>MGSTRLRNASVWLCGLLCLLQVVPSINADVSGCKPGFSSAEYIFSVNRRELERGRKLGKVNFSDCTTRKHGLYDVGDSRFRVLPDGTVLVKRHVKLHKDTKFTISTWDARGIKHSTNIAVASKRHRSGEEAHSRSSKLPVLTFPETHTGLKRKKRDWVIPPIKVSENERGPFPKRLVQIKSNKDRFNKVYYSITGQGADNPPQGVFRIEWETGWMLVTRPLDREEYDKYVLSSHAVSENGSPVEEPMEITINVIDQNDNRPKFTQDVFRGSVREGVQPGTQVMAVSATDEDDNIDSLNGVLSYSILKQDPEEPIPNLFTINRETGVISLIGTGLDREKFPEYTLTVQATDLEGAGLSVEGKAIIQITDANDNAPIFDPKTYTALVPENEIGFEVQRLSVTDLDMPGTPAWQAVYKIRVNEGGFFNITTDPESNQGILTTAKGLDFELRKQYVLQITVENAEPFSVPLPTSTATVTVTVEDVNEAPFFVPAVSRVDVSEDLSRGEKIISLVAQDPDKQQIQKLSYFIGNDPARWLTVNKDNGIVTGNGNLDRESEYVKNNTYTVIMLVTDDGVSVGTGTGTLILHVLDVNDNGPVPSPRVFTMCDQNPEPQVLTISDADIPPNTYPYKVSLSHGSDLTWKAELDSKGTSMLLSPTQ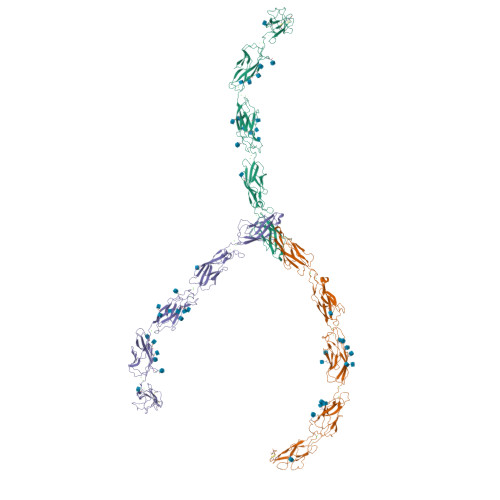QLKKGDYSIYVLLSDAQNNPQLTVVNATVCSCEGKAIKCQEKLVGGFDLPIILVILGSVLALLILFLLLLLFLKRKKVVKEPLLLPEDDTRDNIFYYGEEGGGEEDQDYDLSQLHRGLDSRPDIMRNDVVPTLMPAPHYRPRPSNPDEIGNFIDENLDAADNDPTAPPYDSLLVFDYEGSGSEAASLSSLNSSNSNDEHDYNYLSDWGSRFRKLADMYGGDDDEE[3x]> AVNGKGMNPDYKAYLMAPLKKIPEVTNWETFENDLRWAKQNGFYAITVDFWWGDMEKNGDQQFDFSYAQRFAQSVKNAGMKMIPIISTHQCGGNVGDDCNVPIPSWVWNQKSDDSLYFKSETGTVNKETLNPLASDVIRKEYGELYTAFAAAMKPYKDVIAKIELSGGPAGELRYPSYTTSDGTGYPSRGKFQAYTEFAKSKFRLWVLNKYGSLNEVNKAWGTKLISELAILPPSDGEQFLMNGYLSMYGKDYLEWYQGILENHTKLIGELAHNAFDTTFQVPIGAKIAGVHWQYNNPTIPHGAEKPAGYNDYSHLLDAFKSAKLDVTFTCLEMTDKGSYPEYSMPKTLVQNIATLANEKGIVLNGENALSIGNEEEYKRVAEMAFNYNFAGFTLLRYQDVMYNNSLMGKFKDLLGVTPVMQTIVVKNVPTTIGDTVYITGNRAELGSWDTKQYPIQLYYDSHSNDWRGNVVLPAERNIEFKAFIKSKD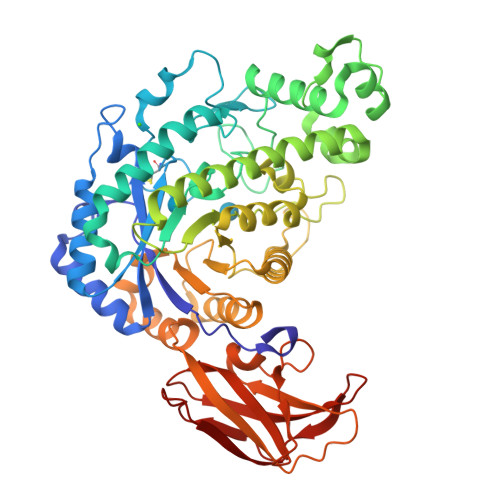GTVKSWQTIQQSWNPVPLKTTSHTSSW> TGAVPRANRIVQQLVEAGADLANIRTMFRNMLRGEEMILSRAEQNVFLQHFPDMLPCG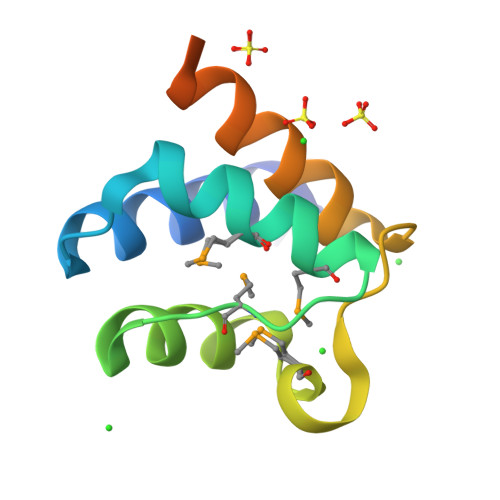IDRNSELAIALREALRRADSQQAARAPARTPPRSSV>[2x]SNAEKEKDTIAAEHKQEASVLLNLHRNKINYLIGETMARMTSLSIAIDR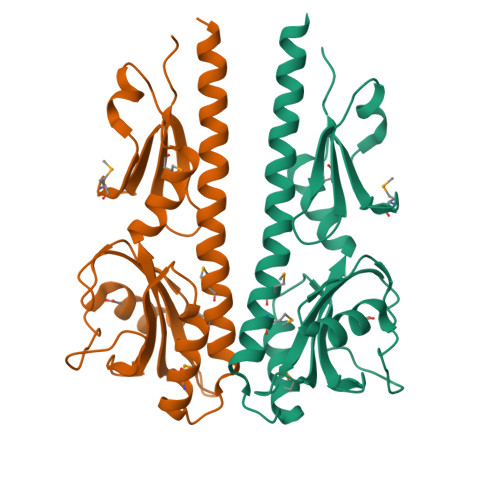PVDIKKMQSILEKTFDSEPRFSGLYFLNAKGDVTASTTELKTKVNLADASFFIKAKETKKTVISDSYSSRITGQPIFTICVPVLDSKRNVTDYLVAAIQIDYLKNLINLLSPDVYIEVVNQDGKMIFASGQASHAEDQKPVSGYLDDISWNMKVYPNPVTIEELSKSL>SMGAVMGTFSSLQTKQRRPSKDIAWWYYQYQRDKIEDELEMTMVCHRPEGLEQLEAQTNFTKRELQVLYRGFKNECPSGVVNEDTFKQIYAQFFPHGDASTYAHYLFNAFDTTQTGSVKFEDFVTALSILLRGTVHEKLRWTFNLYDINKDGYINKEEMMDIVKAIYDMMGKYTYPVLKEDTPRQHVDVFFQKMDKNKDGIVTLDEFLESCQEDDNIMRSLQLFQNVM[4x];>[4x]MAAGVAAWLPFARAAAIGWMPVANCPMPLAPADKNKRQDELIVLNVSGRRFQTWRTTLERYPDTLLGSTEKEFFFNEDTKEYFFDRDPEVFRCVLNFYRTGKLHYPRYECISAYDDELAFYGILPEIIGDCCYEEYKDRKRENAERLMDDNDSENNQESMPSLSFRQTMWRAFENPHTSTLALVFYYVTGFFIAVSVITNVVETVPCGTVPGSKELPCGERYSVAFFCLDTACVMIFTVEYLLRLFAAPSRYRFIRSVMSIIDVVAIMPYYIGLVMTNNEDVSGAFVTLRVFRVFRIFKFSRHSQGLRILGYTLKSCASELGFLLFSLTMAIIIFATVMFYAEKGSSASKFTSIPASFWYTIVTMTTLGYGDMVPKTIAGKIFGSICSLSGVLVIALPVPVIVSNFSRIYHQNQRADKRRAQKKARLARIRVAKTGSSNAYLHSKRNGLLNEALELTGTPEEEHMGKTTSLIESQHHHLLHCLEKTTNHEFIDEQMFEQNCMESSMQNYPSTRSPSLSSHPGLTTTCCSRRSKKTTHLPNSNLPA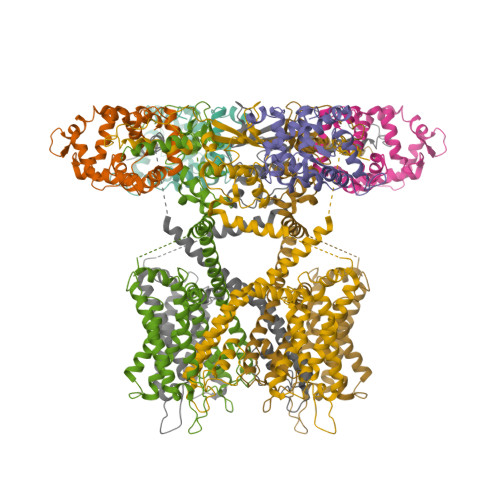TRLRSMQELSTIHIQGSEQPSLTTSRSSLNLKADDGLRPNCKTSQITTAIISIPTPPALTPEGESRPPPASPGPNTNIPSIASNVVKVSAL>[2x]GAMTSWRDKSAKVQVKESELPSSIPAQTGLTFNIWYNKWSQGFAGNTRFVSPFALQPQLHSGKTRGDNDGQLFFCLFFAKGMCCLGPKCEYLHHIPDEEDIGKLALRTEVLDCFG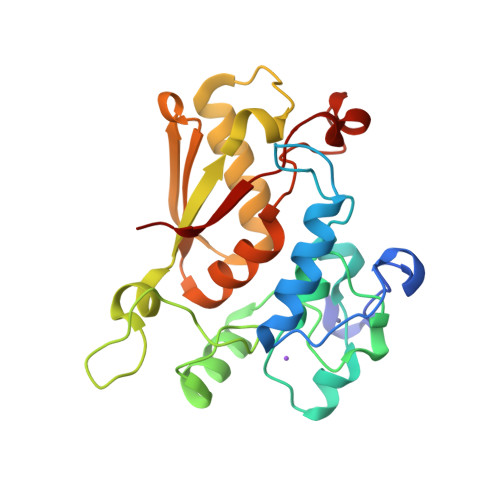REKFADYREDMGGIGSFRKKNKTLYVGGIDGALNSKHLKPAQIESRIRFVFSRLGDIDRIRYVESKNCGFVKFKYQANAEFAKEAMSNQTLLLPSDKEWDDRREGTGLLVKWAN>MRVIFSEDHKLRNAKTELYGGELVPPFEAPFRAEWILAAVKEAGFDDVVAPARHGLETVLKVHDAGYLNFLETAWDRWKAAGYKGEAIATSFPVRRTSPRIPTDIEGQIGYYCNAAETAISPGTWEAALSSMASAIDGADLIAAGHKAAFSLCRPPGHAAGIDMFGGYCFINNAAVAAQRLLDKGAKKIAILDVDFHHGNGTQDIFYERGDVFFASLHGDPAEAFPHFLGYAEETGKGAGAGTTANYPMGRGTPYSVWGEALTDSLKRIAAFGAEAIVVSLGVDTFEQDP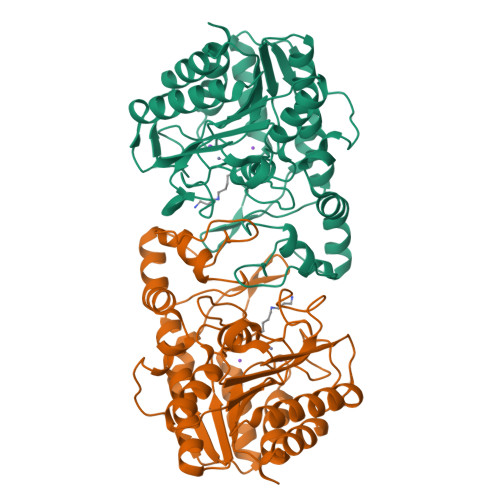ISFFKLTSPDYITMGRTIAASGVPLLVVMEGGYGVPEIGLNVANVLKGVAG[12x]> MVYDLIVIGGGSGGMAAARRAARHNAKVALVEKSRLGGTCVNVGCVPKKIMFNAASVHDILENSRHYGFDTKFSFNLPLLVERRDKYIQRLNNIYRQNLSKDKVDLYEGTASFLSENRILIKGTKDNNNKDNGPLNEEILEGRNILIAVGNKPVFPPVKGIENTISSDEFFNIKESKKIGIVGSGYIAVELINVIKRLGIDSYIFARGNRILRKFDESVINVLENDMKKNNINIVTFADVVEIKKVSDKNLSIHLSDGRIYEHFDH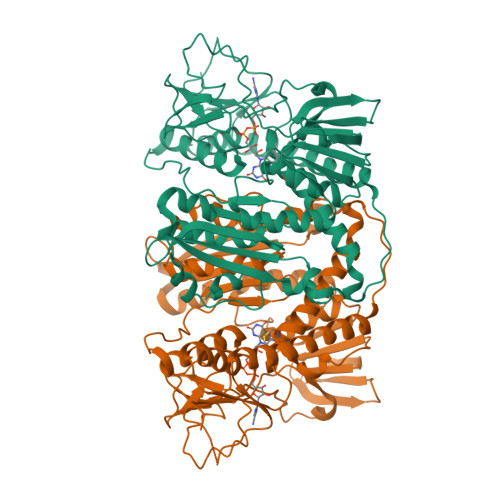VIYCVGRSPDTENLKLEKLNVETNNNYIVVDENQRTSVNNIYAVGDCCMVKKSKEIEDLNLLKLYNEERYLNKKENVTEDIFYNVQLTPVAINAGRLLADRLFLKKTRKTNYKLIPTVIFSHPPIGTIGLSEEAAIQIYGKENVKIYESKFTNLFFSVYDIEPELKEKTYLKLVCVGKDELIKGLHIIGLNADEIVQGFAVALKMNATKKDFDETIPIHPTAAEEFLTLQPWMK> GVMTDVHRRFLQLLMTHGVLEEWDVKRLQTHCYKVHDRNATVDKLEDFINNINSVLESLYIEIKRGVTEDDGRPIYALVNLATTSISKMATDFAENELDLFRKALELIIDSETGFASSTNILNLVDQLKGKKMRKKEAEQVLQKFVQNKWLIEKEGEFTLHGRAILEMEQYIRETYPDAVKICNICHSLLIQGQSCETCGIRMHLPCVAKYFQSNAEPRCPHCNDYWPHEIPKVFDPE;> GPRSQKQLELKVSELVQFLLIKDQKKIPIKRADILKHVIGDYKDIFPDLFKRAAERLQYVFGYKLVELEPKSNTYILINTLEPVEEDAEMRGDQGTPTTGLLMIVLGLIFMKGNTLKETEAWDFLRRLGVYPTKKHLIFGDPKKLITEDFVRQRYLEYRRIPHTDPVDYEFQWGPRTNLELSKMKVLKFVAKVHNQDPKDWPAQYCEALADEENRAR

All MAGE family members contain a shared core MAGE homology domain (MHD) which is a ~ 200 amino acid long domain, which is well conserved across the entire MAGE family (individual human MHD’s share more than 40% sequence identity). The MHD domain structure consists of two highly modified winged helix WH domains WH1 and WH2 in a tandem arrangement linked by an extended β-hairpin. The biochemical basis for this activity appears to be exerted through binding to and modulating the activities of RING domain containing E3 ubiquitin ligases. Rather, each MAGE protein appears to recognize a unique region on its RING partner, suggesting that MAGE proteins are able to function as a versatile and adaptable protein interaction module.

We have noted while examining the MAGE-G1 NSE-1 complex structure that the linker region connecting WH1 and WH2 was absent from the model and the electron density in this region was poor. As the missing residues lie close to a crystallographic 2-fold symmetry axis, the termini of the various domains are positioned such that there are two alternative ways to connect them. To investigate which of these two possibilities is correct, and in the absence of other experimental information, we have downloaded the structure factors and performed a re-refinement of the structure, testing if the data support the alternative connectivity. Our re-refined model has slightly improved refinement and geometry statistics, and we were able to correct a number of minor model building errors in the original coordinates. Electron density maps covering the connecting region, (calculated omitting contributions from residues in the linker region) show significant positive density features generally supporting the alternative connection, although we were unable to completely connect the two domains in this way with 2 residues (163 and 164) being absent from the re-refined model. Importantly for the biological interpretation of the interaction between MAGE-G1 and NSE-1 (and MAGE RING interfaces in general), the re-refined interface between NSE-1 and MAGE-G1 contains contributions from both the N and C-terminal WH domains. In the new interface the N-terminal WH domain of NSE-1 is sandwiched between the two WH domains of MAGE-G1 with additional contacts coming from residues in the linker region and the C-terminal WH domain WHB, some of which involve residues in the second WH domain of NSE-1. Analysis of the interface by the PISA software identified an additional 385 Å2 of interface area (1385 Å2 total), 11 additional hydrogen bonds and 7 additional salt bridges. Support for this interpretation comes from the fact that the in vitro protein-protein interaction data found that both the N and C terminal WH domains of MAGE-G1 were required for NSE-1 binding.> MSSLSRELVFLILQFLDEEKFKETVHKLEQESGFFFNMKYFEEKVHAGEWDEVEKYLSGFTKVDDNRYSMKIFFEIRKQKYLEALDRHDRAKAVDILVKDLKVFSTFNEEAYKEITQLL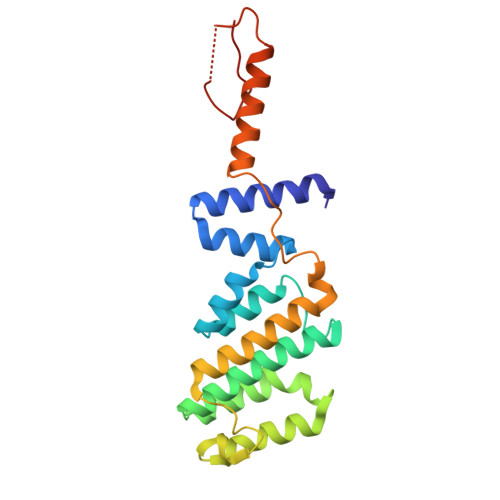TLENFRENEQASKYGDTKSARSIMLIELKKLIEANPLFREKLVFPTLKASRLRTLINQSLNWQHQLCKNPRPNPDIKTLFTDHTCTPPNG> XRTT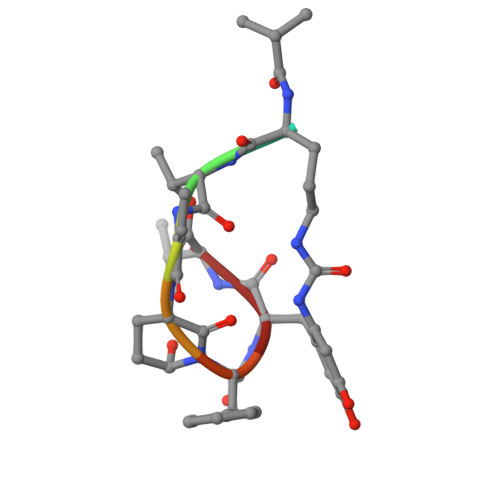EFYV> MSTTLAIVRLDPGLPLPSRAHDGDAGVDLYSAEDVELAPGRRALVRT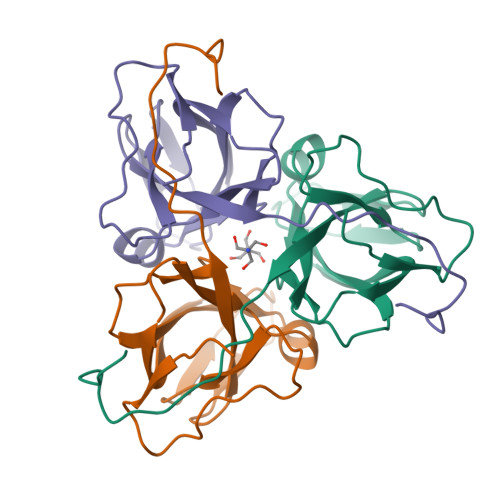GVAVAVPFGMVGLVHPRSGLATRVGLSIVNSPGTIDAGYRGEIKVALINLDPAAPIVVHRGDRIAQLLVQRVELVELVEVSSFDEAGLASTSRGDGGHGSSGGHASL> MKQKVVSIGDINVANDLPFVLFGGMNVLESRDLAMRICEHYVTVTQKLGIPYVFKASFDKANRSSIHSYRGPGLEEGMKIFQELKQTFGVKIITDVHEPSQAQPVADVVDV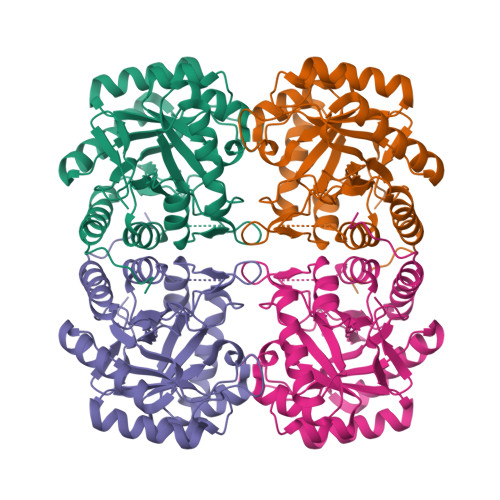IQLPAFLARQTDLVEAMAKTGAVINVKKPQFVSPGQMGNIVDKFKEGGNEKVILCDRGANFGYDNLVVDMLGFSIMKKVSGNSPVIFDVTHALQCRDPFGAASGGRRAQVAELARAGMAVGLAGLFIEAHPDPEHAKCDGPSALPLAKLEPFLKQMKAIDDLVKGFEELDTSK>[2x]SNAMSPISEPSRLDPVRPGQLLMIDLPGPELDKDTAAYLREHGIGAVCLFGKNVESAEQLRRLCADLREVMGEHALIAIDHEGGAITRPEFWPFAPSAMSLGAADDQQLTEDVNAALARQLRSVGINWNFTPVLDINVNPANPVIGDRAYGSDAARVTRHGRAALAGHTREGVAPCAKHF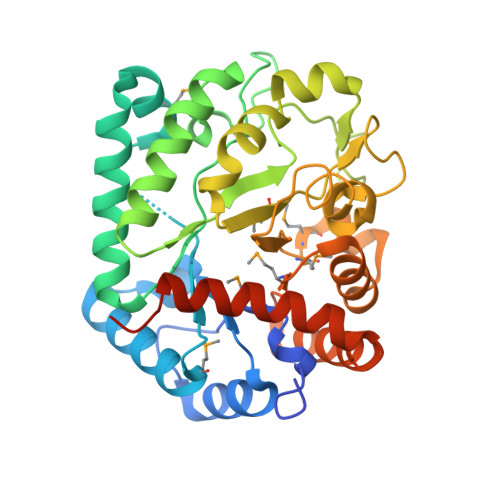PGHGDTHQDSHLALPRVSKSRAELDAGELAPFRALLPETPAIMTAHIVYDALDAEHPATLSPRILTGLLREEWGYDGVIVTDSMGMQAIDANYGRGEAAVRALRAGADLVMALGRREVQQATLAAVAEYVPENQAAVATKRERLRALARRFPAQADETLDPQADAALLADA> AAPTATVTPSSGLSDGTVVKVAGAGLQAGTAYWVAQWARVDTGVWAYNPADNSSVTADANGSASTSLTVRRSFEGFLFDGTRWGTVD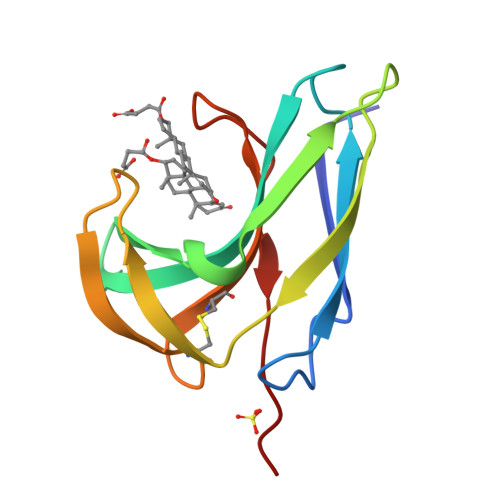CTTAACQVGLSDAAGNGPEGVAISFNHH> GPGSMMQEKILSELAYLRQSIDNFDITLIHILAERFRCTQAIGRLKARYNLPAVDPLREQYQIKRLRKLAIDTHFDPDFAEKFLKFIIKEVVHQHEVIAEKQKIKKENLN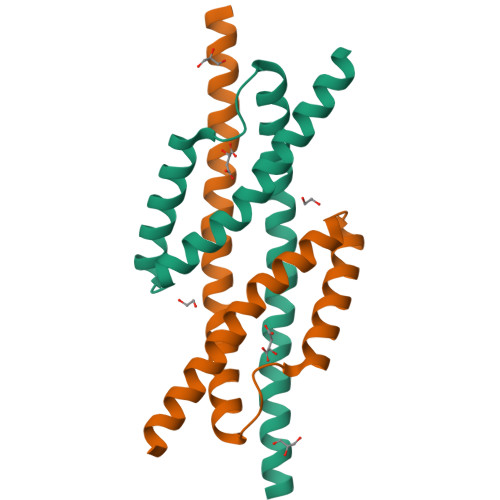ESQN> MNVTIYDVAREASVSMATVSRVVNGNPNVKPSTRKKVLETIERLGYRPNAVARGLASKKTTTVGVIIPDISNIFYAELARGIEDIASMYKYNIILSNSDQNQDKQLHLLNNMLGKQVDGIIFMSGNVTEEHVEELKKSPVPVVLAASIESTNQIPSVTIDYEQAAFDAVQSLIDSGHKNIAFVSGTLEEPINHAKKVKGYKRALTESGLPVRDSYIVEGDYTYDSGIEAVEKLLEEDEKPTAIFVGTDEMALGVIHGAQDRGLNVPNDLEIIGFDNTRLSTMVRPQLTSV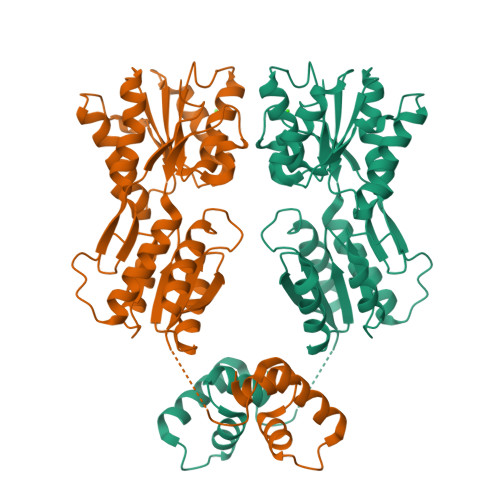VQPMYDIGAVAMRLLTKYMNKETVDSSIVELPHRIEFRQSTK> MLDELVKKELSEEEITEIKLEEIIKYITLIKKSKTFVSSEIRKEELKFLSELAESLFELRLSKVLEGKVGKGFDEFIFDIFKILKQFYVDL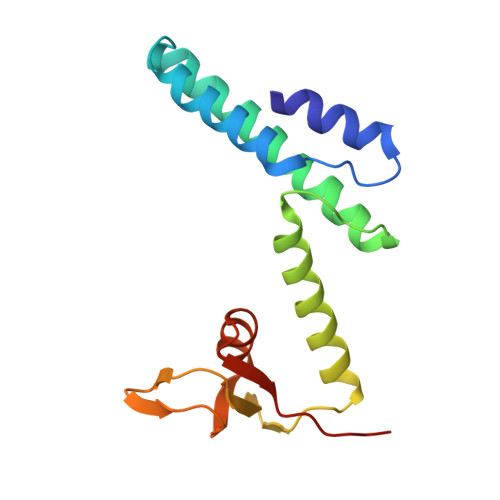LTGRYIIYNDKIYCIVQKPLIYNDHRVNEGDVLVLPMREALPLIIASYLTPYKIDIEEQL> MAKQRVFIAGHRGMVGSAIRRQLEQRGDVELVLRTRDELNLLDSRAVHDFFASERIDQVYLAAAKVGGIVANNTYPADFIYQNMMIESNIIHAAHQNDVNKLLFLGASCIYPKLAKQPMAESELLQGTLEPTNEPYAIAKIAGIKLCESYNRQYGRDYRSVMPTNLYGPHDNFHPSNSHVIPALLRRFHE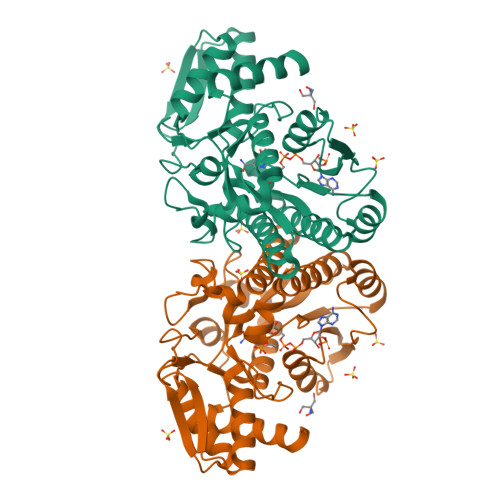ATAQSAPDVVVWGSGTPMREFLHVDDMAAASIHVMELAHEVWLENTQPMLSHINVGTGVDCTIRELAQTIAKVVGYKGRVVFDASKPDGTPRKLLDVTRLHQLGWYHEISLEAGLASTYQWFLENQDRFRG> EVANPEHYIKHPLQNRWALWFF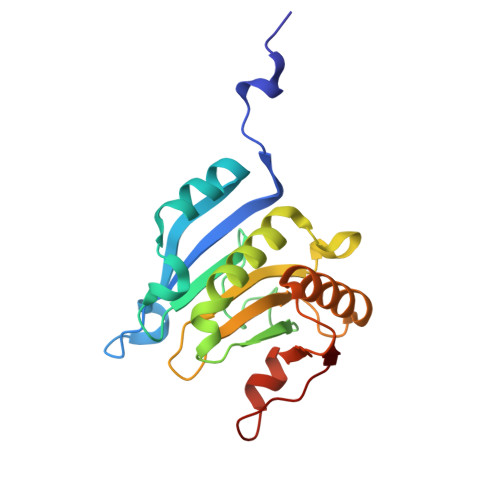KNDKSKTWQANLRLISKFDTVEDFWALYNHIQLSSNLMPGCDYSLFKDGIEPMWEDEKNKRGGRWLITLNKQQRRSDLDRFWLETLLCLIGESFDDYSDDVCGAVVNVRAKGDKIAIWTTECENREAVTHIGRVYKERLGLPPKIVIGYQSHADTATKSGSTTKNRFVV> MKELIYIEEPSILFAHGQKCTDPRDGLALFGPLNQIYGIKSGVVGTQKGLQIFKSYLDKIQKPIYNHNNITRPMFPGFEAVFGCKWESQNIVFKEITDEEIRRYLFNASTHKRTYDLVTLFNDKIITANKNDEERVDVWFVIVPEEIYKYCRPNSVLPNELVQTKSLISKSKAKSFRYTPTLFEEFNKKLKEVEKEAKTYNYDAQFHDQLKARLLEHTIPTQILRESTLAWRDFKNTFGAPIRDFSKIEGHLAWTISTAAYYKAGGKPWKLGDIRPGVCYLGLVYKKIEKSKNPQNACCAAQMFLDNGDGTVFKGEVGPWYNPEKGEYHLKPKEAKALLTQALESYKEQNKSYPKEVFI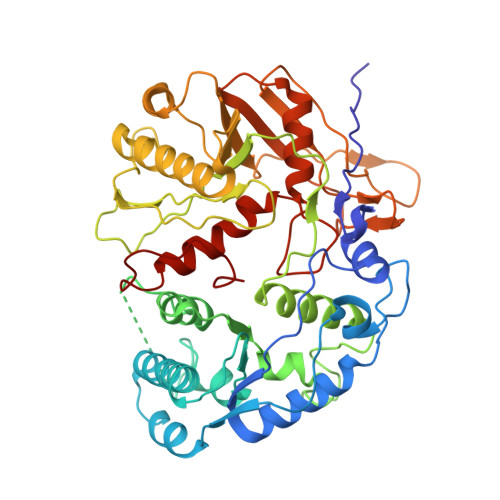HARTRFNDEEWNAFNEVTPKNTNLVGVTITKSKPLKLYKTEGAFPIMRGNAYIVDEKKAFLWTLGFVPKLQSTLSMEVPNPIFIEINKGEAEIQQVLKDILALTKLNYNACIYADGEPVTLRFANKIGEILTASTEIKTPPLAFKYYI> MKGYIQTVTGPVKKADMGLTLPHEHLFNDLSGVVDEPFYEFSHVLVDKKVSADIQWGLKYDPYCCCDNMDKKPIEDVIFELNNFKELGGKTIVDATGSSSIGRDIRKLKQVAELTGINVVASSGLYIEKFEGKRLADDIDAMAKMIDDELNIGIDGTDIRAGMIGEIGVSPFFTDGEKNSLRAAALAQNNNPYASMNIHMPGWQRRGDEVLDILLTEMGCDPAKISLAHSDPSGKDIDYQCKMLDRGVWLEFDMIGLDISFPKEGAAPSVMDTVEAVATLIERGYGNQIVLSHDVFLKQMWAKNGGNGWGFVPNVFLSLLAQRGIDKTIIDKLCIDNPANLLAAENLY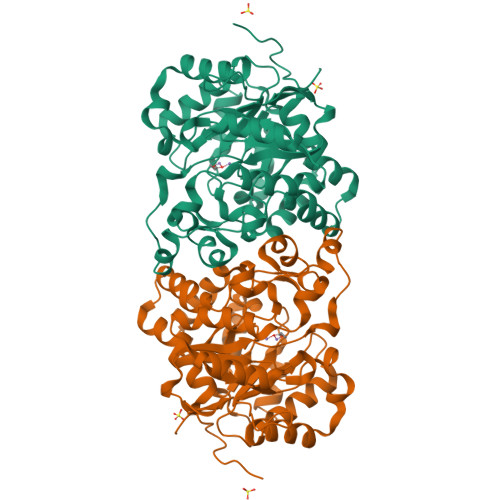FQSHHHHHHWSHPQFEK αHBs are oligomers of 5 or more α-helical peptides that assemble into coiled-coil structures with central solvent-accessible channels. We targeted two properties of αHBs: oligomeric state, which directly affects the internal diameter of the channel; and the identities of channel-facing residues, which fine tune this dimension and introduce different chemistries. The αHBs are loaded with an environment sensitive dye (in this case, 1,6-diphenyl-1,3,5-hexatriene, DPH) that binds within the channels and fluoresces. Accordingly, challenging the array with analytes leads to differential displacement of the dye across the array to give a fluorescent fingerprint.

Despite the requirements for aliphatic residues at a and d, up to 40% of these can be changed to other side chains without compromising barrel integrity. We introduced mutations at one or two of these sites to generate four groups of αHB: Group I had entirely hydrophobic interiors, but with different sizes and shapes of channel; Groups II and III had polar uncharged or polar charged residues, respectively, at specific points along the channel; and Group IV had aromatic residues installed in their channels. The twelve Group III peptides had positively and negatively charged side chains, Lys and Glu, incorporated either singly or paired at a and d sites; and a single peptide with Asp at d. Finally, one third of the designs were crystallized and yielded 12 X-ray crystal structures, all of which were open αHBs with fully accessible channels. Focusing on the small molecules, the αSA signal from the more-polar AAs and CHOs is dominated by the polar and charged Group II and III αHBs.

>XGEIAKALREIAKALREKAYALREIAKALRG[7x]> PISPIETVPVKLKPGMDGPKVAQW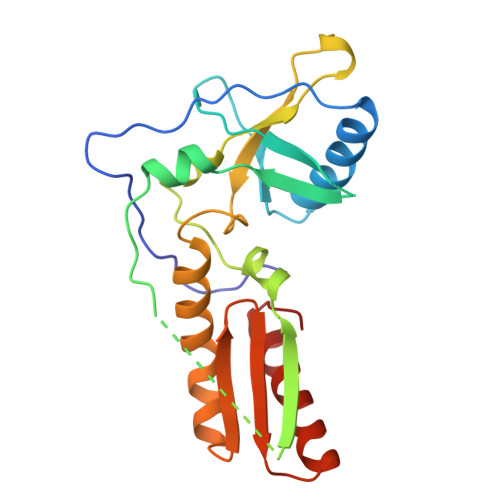PLTAAKIAALVAICTEMEKEGKISKIGPENPYNTPVFAIKKKDSTKWAKLVDFRELNKRTQDFWEVQLGIPHPAGLKKKKSVTVLDVGDAYFSVPLDEDFRKYTAFTIPSINNETPGIRYQYNVLPQGWKGSPAIFQSSMTKILAPFKAANPDIVIYQYMDDLYVGSDLAIGAHRTKIEELRQHLLRWGLTT>[2x]GTKNFIKTWTDRQFLFTLWSWLP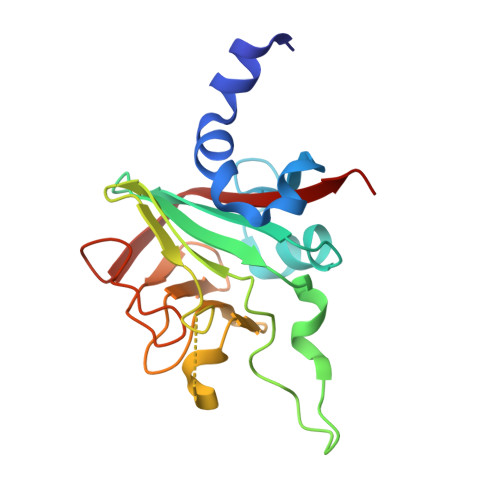VRITMYQPVLLYTTEEHGCSLTTFYVRVEQHEPTLLMIKTCNNEVFGAYCSSRWFERNVKDDKGQRQAYFGTGETFLFSLYPERAKYPWVGIEGDKDLGHSSELFMAADSKMITIGGGEGQAIWMDENIRFGKTDSCKTFNNPPLCPSGDFEIRVLEVYGFVGI> MTSKREKSLDHT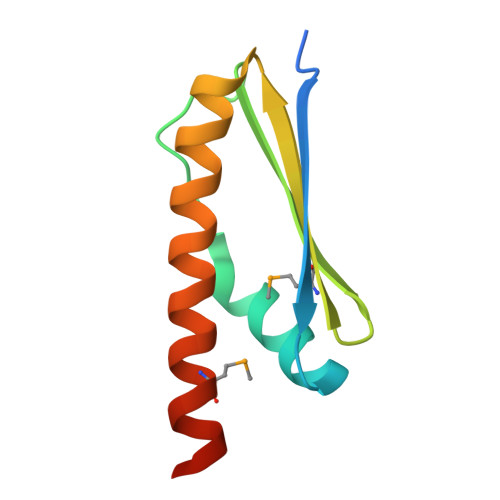LELKIPFETERQATIATKVLSPDPILKPQDFQVDYSSEKNVMLVQFRSIDDRVLRVGVSSIIDSIKTIVEAMDVLSHHHHHH> SSTMIDDEALKEVCEKFECSEEEVLSCLYNRNHQDPLAVAYHLIIDNR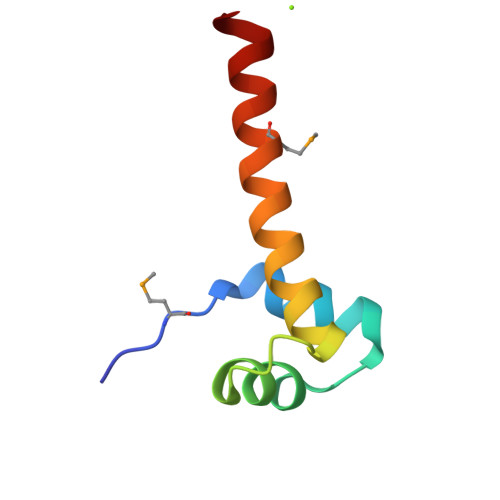RIMNELEHHHHHH The São Paulo MBL (SPM‐1) is widely distributed in South America, Europe and North America, in the Gram‐negative pathogen Pseudomonas aeruginosa. Like other B1 MBLs (NDM, VIM and IMP),10 SPM‐1 has a binuclear zinc center, but has loop characteristics of the B2 MBLs, suggesting it is a B1/B2 hybrid, which, consequently, may be challenging to inhibit. SPM‐1, like other B1 MBLs, has a di‐zinc ion active site with one zinc ion bound at a (normally tetrahedral) tri‐histidine site (Zn1) and one in a trigonal bipyramidal site (Zn2) comprised of conserved Asp, Cys, and His residues. SPM‐1 is distinguished from other B1 MBLs in possessing a “wall” of hydrophobic residues involving Phe57 and Tyr58 on its L3 loop, Phe79 on the loop connecting α5 and α1, and Phe151 and Tyr152 on the kinked α3 helix in the “closed” form, as well as Tyr228 on the opposite side of the active site cleft.

SPM‐1 crystallized in its di‐zinc “closed” form,10a in which the α3 region folds over the active site, and in a previously unreported space group (P4222). The resolution extended to 1.7 Å for uncomplexed crystals and 2.38 Å for inhibitor soaked crystals.

>[2x]GPKSSDHVDLPYNLTATKIDSDVFVVTDRDFYSSNVLVAKMLDGTVVIVSSPFENLGTQTLMDWVAKTMKPKKVVAINTHFHLDGTGGNEIYKKMGAETWSSDLTKQLRLEENKKDRIKAAEFYKNEDLKRRILSSHPVPADNVFDLKQGKVFSFSNELVEVSFPGPAHSPDNVVVYFPKKKLLFGGCMIKPKELGYLGDANVKAWPDSARRLKKFDAKIVIPGHGEWGGPEMVNKTIKVAEKAVGEMRL> WNPPTFSPALLVVTEGDNATFTCSFSNTSESFVLNWYRMSP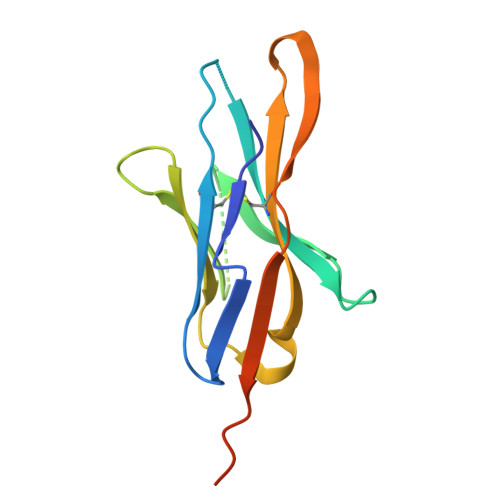SNQTDKLAAFPEDRSQPGQDCRFRVTQLPNGRDFHMSVVRARRNDSGTYLCGAISLAPKLQIKESLRAELRVTERRAEVPTAHPSPSP> GCACCTGTA;> TACACCG;> TGATGTGGTG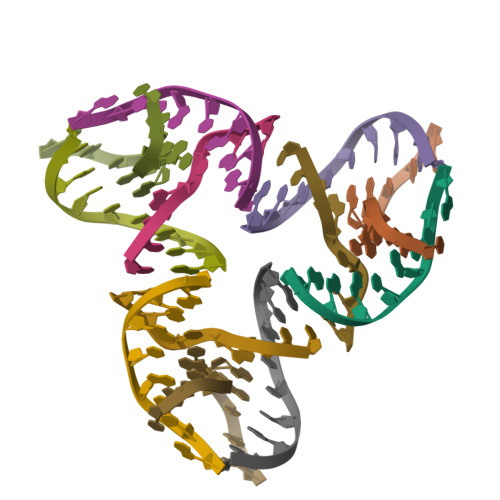C;> CGGACATCA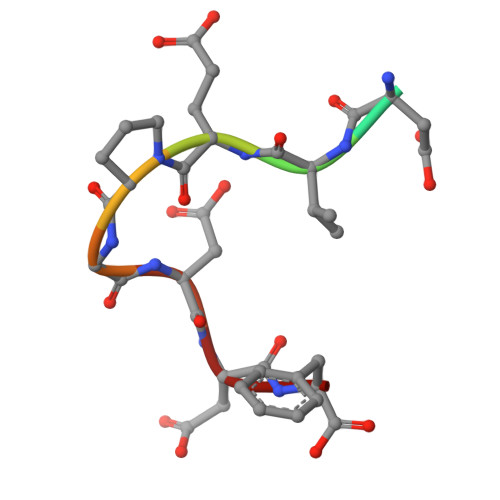> GEDVEPGDDF> MLNQVEVLREEYVEGYVVQMWRRNPSNAPVIEVFTEDNLEEGIIPEYVT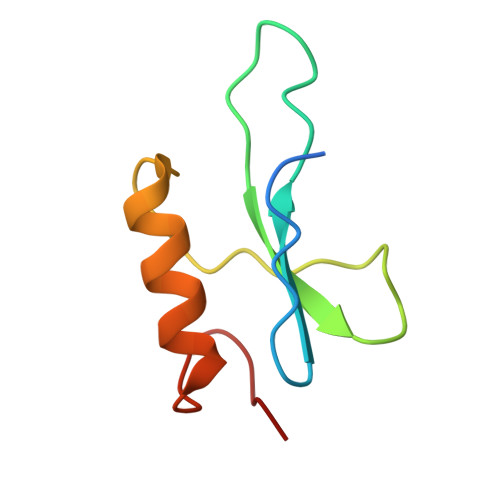ANDDTFDRIVDAVEFGYLEELELV Intramembrane proteases are one class of membrane proteins, which share the property of cleaving transmembrane (TM) proteins to release cytoplasmic, luminal, or extracellular domains that move to new locations where they can carry out their biological functions. Rhomboids, first discovered as part of the epidermal growth factor signalling pathway in Drosophila, are characterised by a core of six TM helices. Structures of the rhomboid protease GlpG from Escherichia coli and Haemophilus influenzae have revealed that the catalytic dyad serine and histidine forms part of a water-filled cavity separated from the external medium by a flexible loop and from the bilayer by TM helices. Substrate proteins are thought to diffuse laterally through gaps between TM helices to reach the rhomboid active site.

The first one was obtained from a completely delipidated protein for the wild-type (WT) protein in a trigonal crystal form (space group, R32) and diffracted to 1.85 Å. The structures of GlpG WT and S201T in this crystal form are largely identical except for a small difference in L5 (rmsd for Cα atoms excluding L5 is 0.15 Å). The hydroxyl of Thr201 points away from active-site His254 and is within hydrogen-bonding distance to the side-chain amide of Asn154 and the imidazole nitrogen of His150, both residues being part of the oxyanion hole, thus explaining the inactivity. The mutation of serine to threonine results in a displacement of side chain of the active-site histidine by ∼ 1 Å. Of the 18 fully or partially ordered detergent molecules in the trigonal crystal form of GlpG S201T, many take similar positions to lipids, binding in grooves and crevices in the protein and demonstrating how the native structure of GlpG is preserved in a detergent environment. Six detergent molecules surround L1 and two occupy the space beneath it, thus preserving the structure of L1. BNG514 observed in the trigonal crystal form occupies the space between TM2/TM5 and protrudes into the active site. Such an insertion of detergent results in minimal structural change involving only a partial displacement of L5 in particular residues (residues 245–247). Glycine and proline are residues that are known to introduce kinks in TM helices, and it is probable that the TM helix of the substrate must bend towards the enzyme thereby juxtaposing the cleavage site of the substrate with the active site of enzyme. This detergent molecule may be mimicking a rhomboid substrate bending towards the active site. A small displacement of L5 lifts the side chains of Phe245 and Met247, but Met249 in the present structure still plugs the cavity near the active site.

> ERAGPVTWVMMIACVVVFIAMQILGDQEVMLWLAWPFDPTLKFEFWRYFTHALMHFSLMHILFNLLWWWYLGGAVEKRLGSGKLIVITLISALLSGYVQQKFSGPWFGGLTGVVYALMGYVWLRGERDPQSGIYLQRGLIIFALIWIVAGWFDLFGMSMANGAHIAGLAVGLAMAFVDSLN> GSTSARNHTEDNSTEYYDYEEARSACPARHLNNTNGTVLKLLG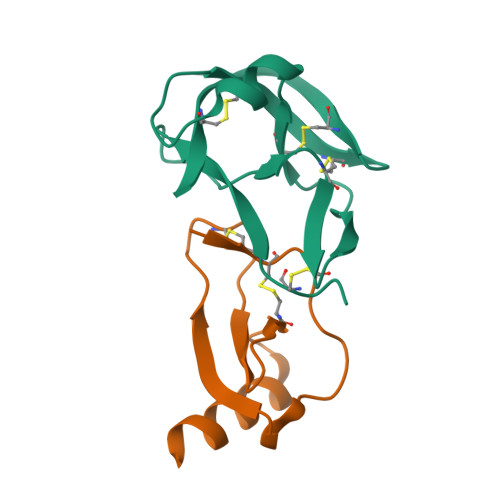CHYFCNGTLSTAPDGYPCYNLTAQQVRTLTTYPNTSCAVGVCMKGTCVKNGTMEQCFKTP;> ARGTNVGRECCLEYFKGAIPLRKLKTWYQTSEDCSRDAIVFVTVQGRAICSDPNNKRVKNAVKYLQSLERS>[2x]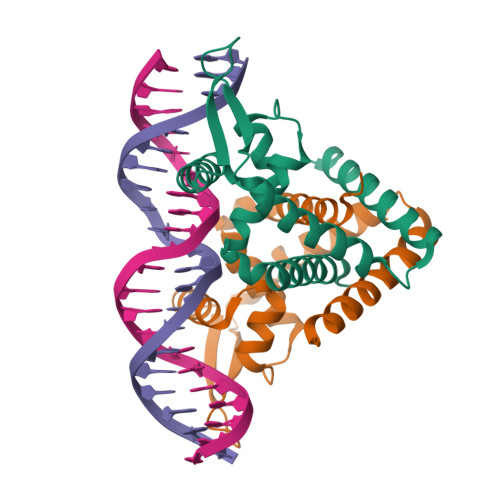MESTLGSDLARLVRVWRALIDHRLKPLELTQTHWVTLYNINRLPPEQSQIQLAKAIGIEQPSLVRTLDQLEEKGLITRHTSANDRRAKRIKLTEQSSPIIEQVDGVISSTRKEILGGISSDEIAVLSGLIDKLEKNIIQLQTKLEHHHHHH Here we report that histones are major chromatin components in the bacteria Bdellovibrio bacteriovorus and Leptospira interrogans. Crystal structures (<2.0 Å) of the B. bacteriovorus histone (Bd0055) dimer and the histone–DNA complex confirm conserved histone-fold topology but indicate a distinct DNA-binding mode. Unlike known histones in eukaryotes, archaea and viruses, Bd0055 binds DNA end-on, forming a sheath of dimers encasing straight DNA rather than wrapping DNA around their outer surface. The bacterial histone Bd0055 from B. bacteriovorus HD100 is structurally similar to its archaeal and eukaryotic homologues but, rather than wrapping DNA around its outer surface, binds DNA edge-on and oligomerizes to form a dense nucleohistone fibre that completely encases DNA in vitro.

We solved the crystal structure of Bd0055 to 1.8 Å resolution. Bd0055 forms a crystallographic dimer where one monomer is related to its partner through two-fold symmetry. It has the overall topology of a histone-fold dimer, as well as a positively charged ridge along its ‘top’ surface that is also found in archaeal and eukaryotic histones, where it is used for DNA binding. Of note, the Bd0055 α2 helix is 7 Å shorter than its archaeal and eukaryotic histone counterparts (1 helical turn shorter compared with archaeal HMfB), which decreases the overall size of the histone dimer. In addition, the α3 helix in Bd0055 forms only one helical turn and the remaining amino acids pack against α2 of the dimerization partner in an extended configuration. This organization differs from the three-turn α3 helix in archaeal/eukaryotic histones, which takes part in tetramerization by contributing to the four-helix bundle interface. A conserved histidine in α2 (H49) is conspicuously absent from bacterial histones. Finally, the surface opposite the basic ridge of the Bd0055 dimer is more acidic than that of HMf/HTk histones.

> MAEVLVVTSKVKKLIKEKGQMNTSAETIDVLSKAIEQLCLKGVESAKADGRKTVMARDIVIDHL>MFADLDYDIEEDKLGIPTVPGKVTLQKDAQNLIGISI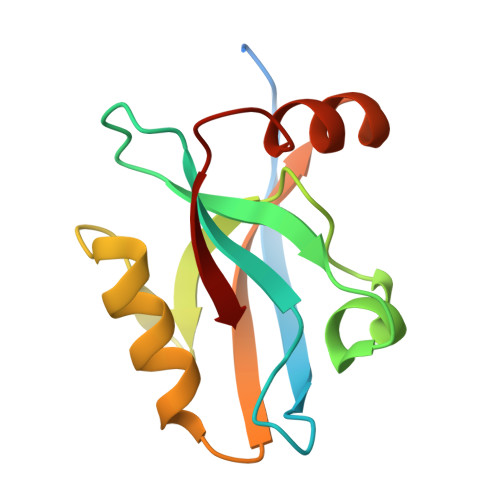GGGAQYCPCLYIVQVFDNTPAALDGTVAAGDEITGVNGRSIKGKTKVEVAKMIQEVKGEVTIHYNKLQADPKQLEVLFNGPGIESVKI[2x]Here structural analysis of hydroxyketoacid aldolase from Sphingomonas wittichii RW1 (SwHKA) revealed a dynamic movement of the metal cofactor between two coordination spheres without protein scaffold rearrangements. Holo‐SwHKA forms a trimer of homodimers, in which each monomer adopts an (α/β)8 triosephosphate isomerase (TIM) barrel fold. In total, holo‐SwHKA contains six equivalent active sites; each of which is formed from amino acids from two different domain‐swapped dimers. The transition from M2+ R to M2+ A,S is induced by bidentate substrate binding and occurs without a concomitant rearrangement of the protein scaffold.

To investigate a potential structural role for the metal cofactor in the M2+ R configuration through interactions with residue S116′, two different variants were designed at this position. Identical orientations of the alanine/serine residues were observed, and the protein fold was unaffected by the mutation (rmsd=0.115 Å between 230 Cα atoms). In the presence of ketoacids, bidentate substrate coordination affords M2+ A,S as the lowest energy complex and predominant state in crystal structures. For the S116A mutant, a lower apparent K d (i.e. higher affinity) toward M2+ A,S was observed with Mg2+, while the affinity remained mostly unaffected when Mn2+ was used. These data suggest that elimination of M2+ R could remove the competition between the two binding modes, and thereby increase its affinity toward the M2+ A,S configuration.

>[2x]HHNKVRTCWNEGRPALAGWLQLPGTLHAEALARLDYDAVVIDMQHSPIDFGQVAPMLIAIELGGAEPFVRTQVNDPSDIMKLLDAGAYGIIAPMVNTRAEAQTLASALHYSPRGLRAFGPRRPSLRYGSGYLAQASETVVGLAMIETREALANIDEILSVDGIDGVFIGPTDLALDLGHAPLVDTEEAEVVSAIAHVRERAHAAGKRVGIFCGSGGFARVKLAEGFDFVTAAPDLAMLSAAARQVIADARAL1-(2,4-dichlorophenyl)-3-oxidanyl-urea 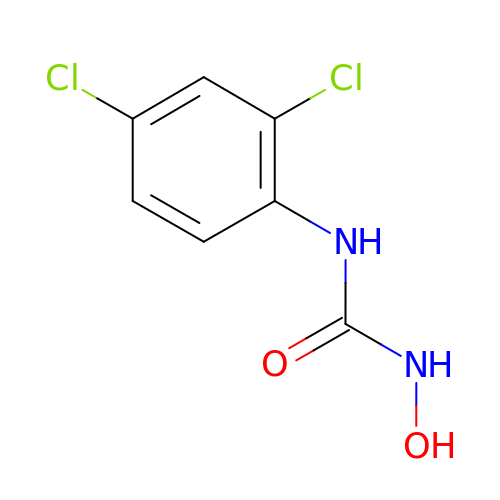| C7 H6 Cl2 N2 O2 | DJPGEWSKXZZHCC-UHFFFAOYSA-N>[2x]LPVDKYPVLKDQPAEVLFRENNPTVLECIIEGNDQGVKYSWKKDGKSYNWQEHNAALRKDEGSLVFLRPQASDEGHYQCFAETPAGVASSRVISFRKTYLIASPAKTHEKTPIEGRPFQLDCVLPNAYPKPLITWKKRL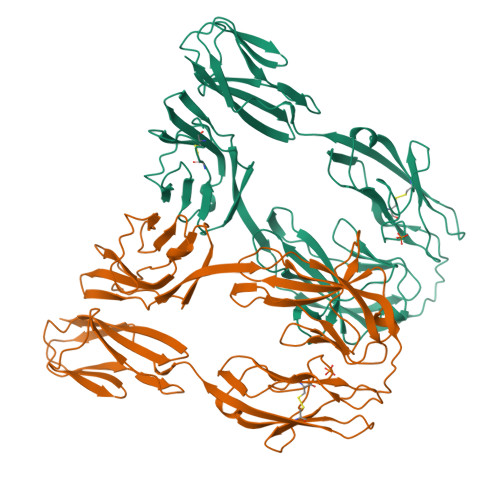SGADPNADVTDFDRRITAGPDGNLYFTIVTKEDVSDIYKYVCTAKNAAVDEEVVLVEYEIKGVTKDNSGYKGEPVPQYVSKDMMAKAGDVTMIYCMYGSNPMGYPNYFKNGKDVNGNPEDRITRHNRTSGKRLLFKTTLPEDEGVYTCEVDNGVGKPQKHSLKLTVVSAPKYEQKPEKVIVVKQGQDVTIPCKVTGLPAPNVVWSHNAKPLSGGRATVTDSGLVIKGVKNGDKGYYGCRATNEHGDKYFETLVQVN> GPLGSDSKIEKMLPDGGRLVVFPN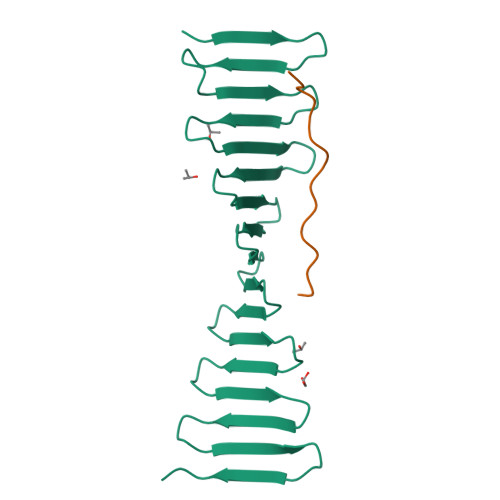GTRKELSADGQTVKVMFFNGDVKHTMPDQRVIYYYAEAQTTHITYPDGMEVLQFPNNQTEKHFPDGRKEITFPDQTVKTLHPDGREESVLTDGTIIQLNPDGSKVIQFNTGQREIHTADFKRREYPDGTVKTVYSDGRQETQYPTGRVRLKDPQGKVIMD;> GPLGSCYQNKLSISDHDSGVEDEDLSPRPSPNPHPVSQQTKRVHPLVPELSMVLDGSFLD> MYFYRRIPSLASKMNHMRQFSLPRSSAAIIMAASTAALAVPCRAMHGKPASGHKVRTQHSRRWWMQSKAHHLTAVPHEEARSRPHFPAYTEDVDQPMVVPDGVCCFNCDKPIDGDDINSYVWVPSGNARVPTTQGYFFHVKCFKCWNCKYRIIHNQFYSKDSRAWCLSCALGRDIRVPTRRWHTSYVNTHRTGS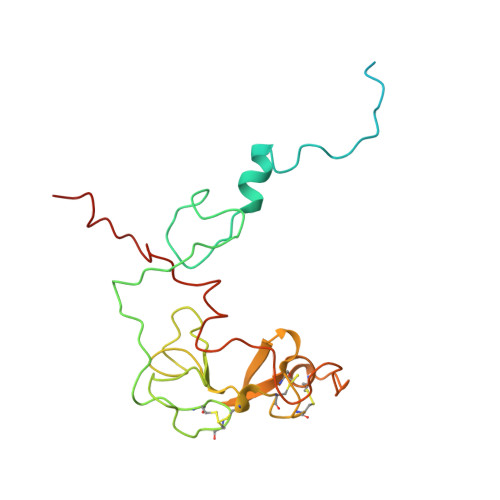RLTGQFFPRHRHQMEFLFSPKE> PSPDELKPFPTVQQTIFRGHEGRVRSVAIDPTGVALATGGDDGTVRVWELLTGRQVWSVKLNGDEAVNTVRWRPTKDTFILAAAAGEDIFLMIPTHPSVTPALDQASRDILNAGFGHATNGKQQANLPPGKEPPGKWARPGTRLEDEGVLLRITVRSTIKAISWHRRGDHFATVSPSGQRSSVAIHTLSKHLTQIPFRKLNGLAQTAS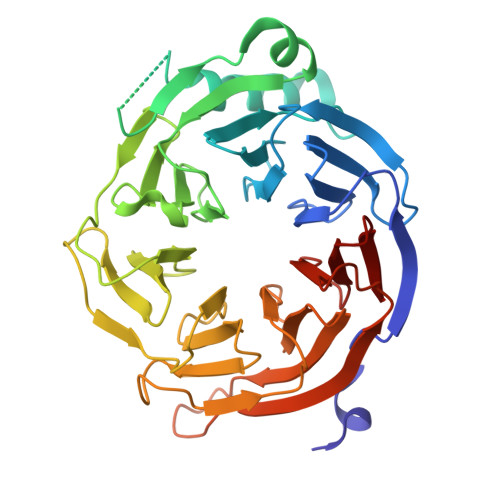FHPLRPLFFVATQRSIRCYDLQKLELVKIVQPGAKWISSFDVHPGGDNLVVGSYDKRLLWHDLDLSNRPYKTMRFHTEAIRAVRFHKGGLPLFADASDDGSLQIFHGKVPNDQLENPTIVPVKMLKGHKVVNKLGVLDIDWHPREPWCVSAGADGTARLWM ferutinine | C22 H30 O4 | 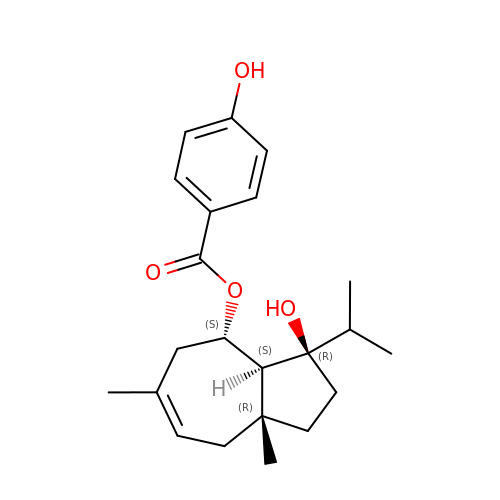CYSHNJQMYORNJI-YUVXSKOASA-N2,6-diethylphenol | C10 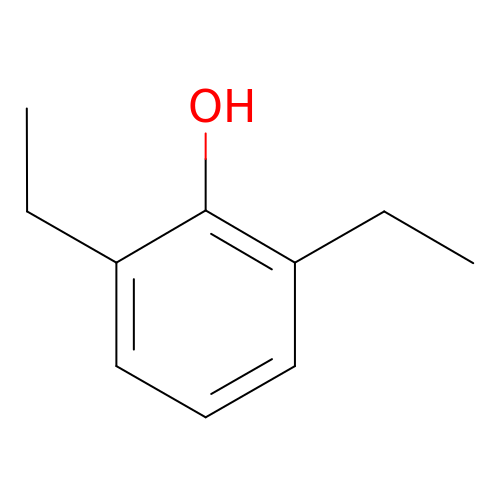H14 O | METWAQRCMRWDAW-UHFFFAOYSA-N> SAAPSVFLIDDDRDLRKAMQQTLELAGFTVSSFASATEALAGLSADFAGIVISDIRMPGMDGLALFRKILALDPDLPMILVTGHGDIPMAVQAIQDGAYDFIAKPFAADRLVQSARRAEKKRRLVMENRSLRRAAEAASE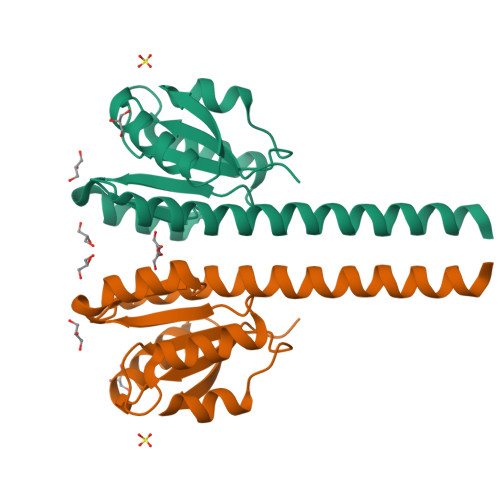GLKLAAALEHHHHHH phenylphosphonic acid | C6 H7 O3 P | 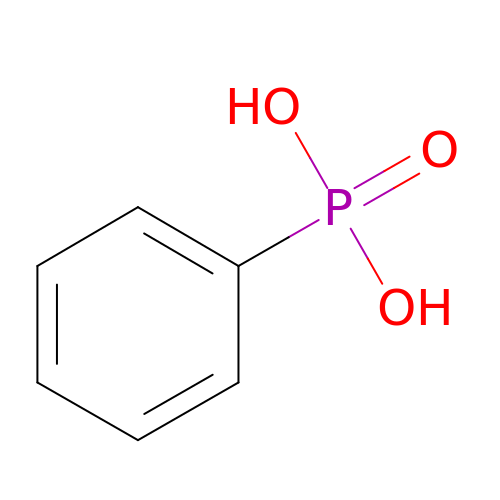QLZHNIAADXEJJP-UHFFFAOYSA-N>AVTGDTDQPI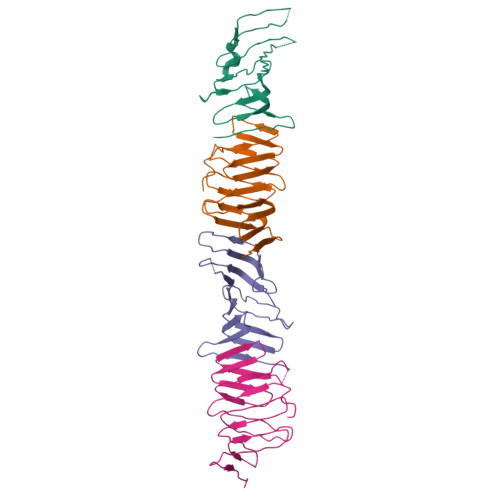HIESDQQSLDMQGNVVTFTGNVIVTQGTIKINADKVVVTRPGGEQGKEVIDGYGKPATFYQMQDNGKPVEGHASQMHYELAKDFVVLTGNAYLQQVDSNIKGDKITYLVKEQKMQAFSDKGKRVTTVLVPSQLQDKNNKGQTPAQKKGN[8x]1-[6-(dimethylamino)naphthalen-2-yl]ethanone 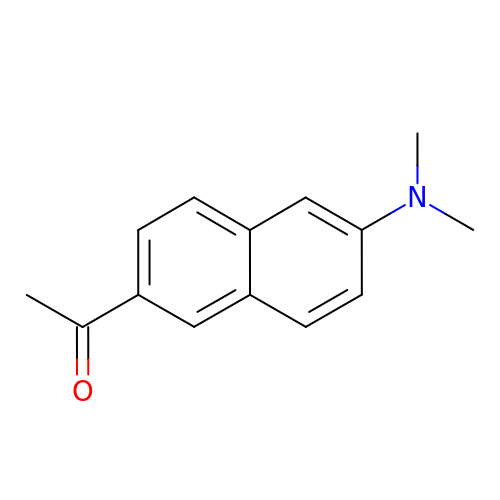| C14 H15 N O | FUVQYVZTQJOEQT-UHFFFAOYSA-N> DQKLNTDLQETFSGFQKQLQSVLETDFFRDDSLMKGAIQMIHSKIMQMLLQSLIPEGLHQDITTDTGSKKSEIRSSDAHRILDLTWKHVHYPIFKYFQNWRNRNVAEGSRPNYAGHRQLNSILQKIFPQIHKLYYSTLELIFANYNLTALIPSDTRSKLNISTKKLNDDASNVLKPEDSFSIDCVMASQRCLLYIGCSQRYKIIMEHLSDRYQQADFQKPLRYLDIASTIVPSVGETFLQRGICYTHTKNFGNAAYQFVRSSLSRLPSDAGIPNFTNLLGDPNGSLFKKLLNSLDDLKVQETIKKRIINMEIME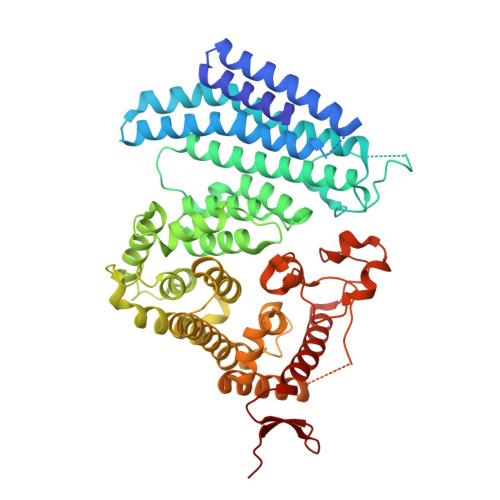FYILPLIGSHIFPQTWKNNRHSDRLKHFQTLLFDKIEIRYIKNISMIFQDLILLIGSFHMYQMINGVSSNIRSIQSETKFLEFIFKFFTHLIDKVIMKEFKNCEMFQYLAMARIMMCWIKSHKNVLKFAHRSTSFCQSMVNLTNELLSSNDLSISFEHLHRPTRDYFYEEDIMLKEFGPTKFTLSDFNDEKLLSMDNLPDRLVGKSKNKLTAKEEHSSRVQVLVYSNKKFLEKNCCGFKLDTEKKRYVHTAVK> MSVDPMTYEAQFFGFTPQTCMLRIYIAFQDYLFEVMQAVEQVILKKLDGIPDCDISPVQIRKCTEKFLCFMKGHFDNLFSKMEQLFLQLILRIPSNILLPEDKCKETPYSEEDFQHLQKEIEQLQEKYKTELCTKQALLAELEEQKIVQAKLKQTLTFFDELHNVGRDHGTSDFRESLVSLVQNSRKLQNIRDNVEKESKRLKIS;> MTISRVKLLDTMVDTFLQKLVAAGSYQRFTDCYKCFYQLQPAMTQQIYDKFIAQLQTSIREEISDIKEEGNLEAVLNALDKIVEEGKVRKEPAWRPSGIPEKDLHSVMAPYFLQQRDTLRRHVQKQEAENQQLADAVLAGRRQVEELQLQVQAQQQAWQALHREQRELVAVLREPE;> MSHQERLQSKSLHLSPQEQSASYQDRRQSWRRASMKETNRRKSLHPIHQGITELSRSISVDLAESKRLGCLLLSSFQFSIQKLEPFLRDTKGFSLESFRAKASSLSEELKHFADGLETDGTLQKCFEDSNGKASDFSLEASVAEMKEYITKFSLERQTWDQLLLHYQQEAKEILSRGSTEAKITEVKVEPMTYLGSSQNEVLNTK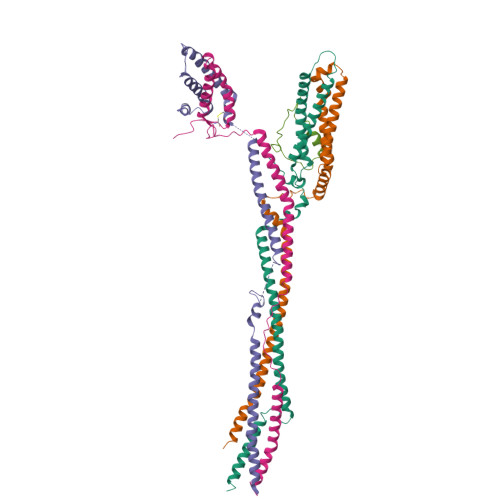PDYQKILQNQSKVFDCMELVMDELQGSVKQLQAFMDESTQCFQKVSVQLGKRSMQQLDPSPARKLLKLQLQNPPAIHGSGSGSCQHHHHHH;> MAGSPELVVLDPPWDKELAAGTESQALVSATPREDFRVRCTSKRAVTEMLQLCGRFVQKLGDALPEEIREPALRDAQWTFESAVQENISINGQAWQEASDNCFMDSDIKVLEDQFDEIIVDIATKRKQYPRKILECVIKTIKAKQEILKQYHPVVHPLDLKYDPDPAPHMENLKCRGETVAKEISEAMKSLPALIEQGEGFSQVLR;> GPLGSMAASGLDHLKNGYRRRFCRPSRARDINTEQGQNVLEILQDCFEEKSLANDFSTNSTKSVPNSTRKIKDTCI> MKAETKSYKMDDGKTVDIPKDPKRIAVVAPTYAGGLKK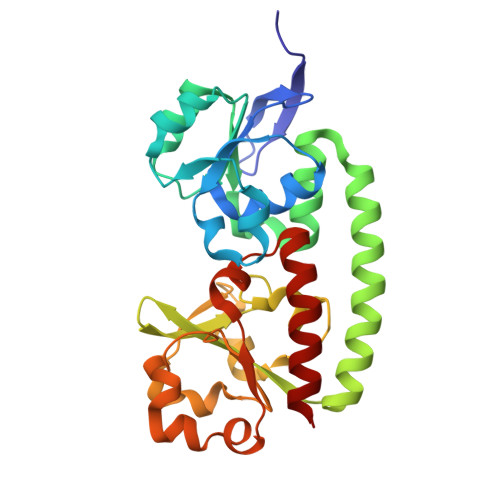LGANIVAVNQQVDQSKVLKDKFKGVTKIGDGDVEKVAKEKPDLIIVYSTDKDIKKYQKVAPTVVVDYNKHKYLEQQEMLGKIVGKEDKVKAWKKDWEETTAKDGKEIKKAIGQDATVSLFDEFDKKLYTYGDNWGRGGEVLYQAFGLKMQPEQQKLTAKAGWAEVKQEEIEKYAGDYIVSTSEGKPTPGYESTNMWKNLKATKEGHIVKVDAGTYWYNDPYTLDFMRKDLKEKLIKAAK>MPSLMSFGSCQWIDQGRFSRSLYRNFKTFKLHEMHGLCMPNLLLNPDIHGDRIIFVCCDDLWEHDLKSGSTRKIVSNLGVINNARFFPDGRKIAIRVMRGSSLNTADLYFYNGENGEIKRITYFSGKSTGRRMFTDVAGFDPDGNLIISTDAMQPFSSMTCLYRVENDGINFVPLNLGPATHILFADGRRVIGRNTFELPHWKGYRGGTRGKIWIEVNSGAFKKIVDMSTHVSSPVIVGHRIYFITDIDGFGQIYSTDLDGKDLRKHTSFTDYYPRHLNTDGRRILFSKGGSIYIFNPDTEKIEKIEIGDLESPEDRIISIPSKFAEDFSPLDGDLIAFVSRGQAFIQDVSGTYVLKVPEPLRIRYVRRGGDTKVAFIHGTREGDFLGIYDYRTGKAEKFEENLGNVFAMGVDRNGKFAVVANDRFEIMTVDLETGKPTVIERSREAMITDFTISDNSRFIAYGFPLKHGETDGYVMQAIHVYDMEGRKIFAATTENSHDYAPAFDADSKNLYYLSYRSLDPSPDRVVLNFSFEVVSKPFVIPLIPGSPNPTKLVPRSMTSEAGEYDLNDMYKRSSPINVDPGDYRMIIPLESSILIYSVPVHGEFAAYYQGAPEKGVLLKYDVKTRKVTEVKNNLTDLRLSADRKTVMVRKDDGKIYTFPLEKPEDERTVETDKRPLVSSIHEEFLQMYDEAWKLARDNYWNEAVAKEISERIYEKYRNLVPLCKTRYDLSNVIVEMQGEYRTSHSYEMGGTFTDKDPFRSGR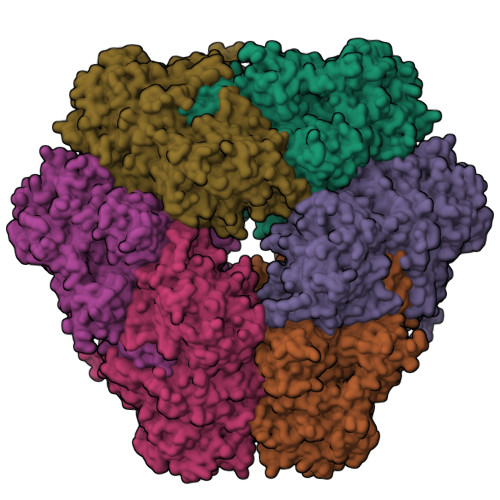IACDFKLDGDHYVVAKAYAGDYSNEGEKSPIFEYGIDPTGYLIEDIDGETVGAGSNIYRVLSEKAGTSARIRLSGKGGDKRDLMIDILDDDRFIRYRSWVEANRRYVHERSKGTIGYIHIPDMGMMGLNEFYRLFINESSYQGLIVDVRFNGGGFVSQLIIEKLMNKRIGYDNPRRGTLSPYPTNSVRGKIIAITNEYAGSDGDIFSFSFKKLGLGKLIGTRTWGGVVGITPKRRLIDGTVLTQPEFAFWFRDAGFGVENYGVDPDVEIEYAPHDYLSGKDPQIDYAIDALIEELRNWNEELPQRPS[6x];>[6x]DQTQKAAAELTFFX> MAQINVIGQNGGRTIELPLPEVNSGVLHEVVTWQLASRRRGTASTRTRAQVSKTGRKMYGQKGTGNARHGDRSVPTFVGGGVAFGPKPRSYDYTLPRQVRQLGLAMAIASRQEGGKLVAVD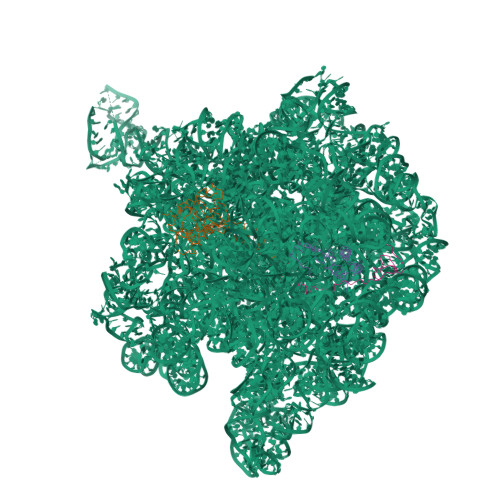GFDIADAKTKNFISWAKQNGLDGTEKVLLVTDDENTRRAARNVSWVSVLPVAGVNVYDILRHDRLVIDAAALEIVEEEAGEEQQ;> MTAPEQTFRNKKQRKQQVKLRKPGFAVAKYVRMSPRKVRLVVDVIRGKSVQDAEDLLRFIPRSASEPVAKVLNSAKANALHNDEMLEDRLFVKEAYVDAGPTLKRLIPRARGSANIIKKRTSHITIIVAEKGNK;> MAKHPVPKKKTSKSKRDMRRSHHALTAPNLTECPQCHGKKLSHHICPNCGYYDGRQVLAV> GGSSQKQMSKKMNDQLELMESNIRRDIRQGFVDLQTEKSDLIDNVGAIPFLDYKHFASRIFFPEAGTLTAVMIRDIGEDSEQTTVDEKCLAFAELIRDKQFLSCFVHALEEQKNFSIKDKCTVASLLTLALHGDLLYLT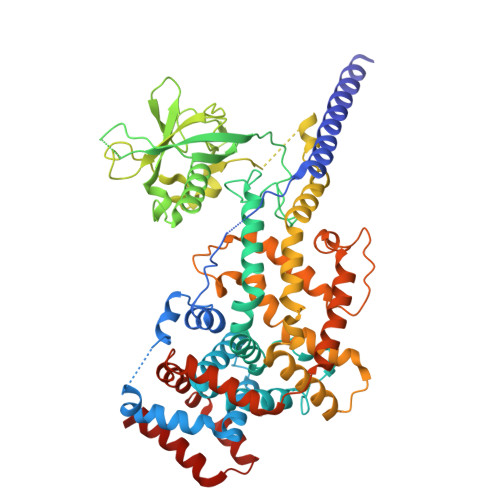EIMEDLLQSLMDQSSNANPKLLLRRTESIVEKLLTNWMSICLYGFLRESVGQPLFLLVSALTQQISKGPVDSVTEKALYTLSEDWLLCQAQDFEPLKLKVVFAVGTGEEISESLEVIALTCDTIQQVKEKILQTFQRKFGFRYTQQIRDIEIEYEKEGKFVMLQEVDDTSEIRGHVTMLNTLKHYQVGDGACIKVITPKIHAPLKTQNSVKDDKNFSIKYFHLVDPDIDTDLSNHPEKKALKIKEMYLIKLLSTKVAVHSFVENLFKSIWGLPNNKAPLAVKYFFDFLDEQAERKKITDPDVLHIWKTNSLPLRFWVNILKNPDFVFSDMEKSPHLDGCLSVIAQAFMDSFSLTDTHLDKHSPTNKLLYGKDIPQYKQEVKSYYKLVKDQTSISSQELKTFLQEESKKHQNEFNESAALRELYKYMQRYFTEIFQKLEQTDAPSNLKENMHRVKELFDNM> SEMASEIHMTGPMCLIENTNGRLMANPEALKILSAITQPMVVVAIVGLYRTGKSYLMNKLAGKKKGFSLGSTVQSHTKGIWMWCVPHPKKPGHILVLLDTEGLGDVEKGDNQNDSWIFALAVLLSSTFVYNSIGTINQQAMDQLYYVTELTHRIRSKSSPDENENEVEDSADFVSFFPDFVWTLRDFSLDLEADGQPLTPDEYLTYSLKLKKGTSQKDETFNLPRLCIRKFFP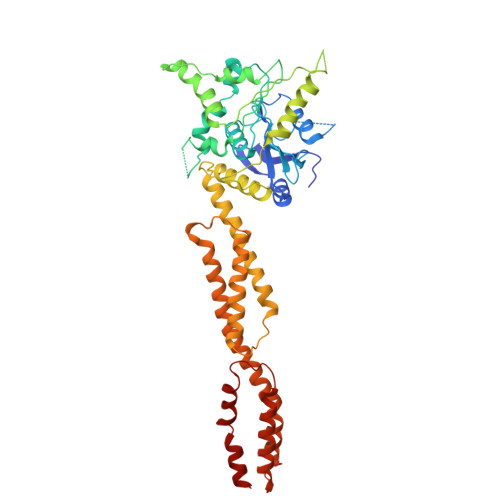KKKCFVFDRPVHRRKLAQLEKLQDEELDPEFVQQVADFCSYIFSNSKTKTLSGGIQVNGPRLESLVLTYVNAISSGDLPCMENAVLALAQIENSAAVQKAIAHYEQQMGQKVQLPTETLQELLDLHRDSEREAIEVFIRSSFKDVDHLFQKELAAQLEKKRDDFCKQNQEASSDRCSALLQVIFSPLEEEVKAGIYSKPGGYRLFVQKLQDLKKKYYEEPRKGIQAEEILQTYLKSKESMTDAILQTD> MPRYAMAID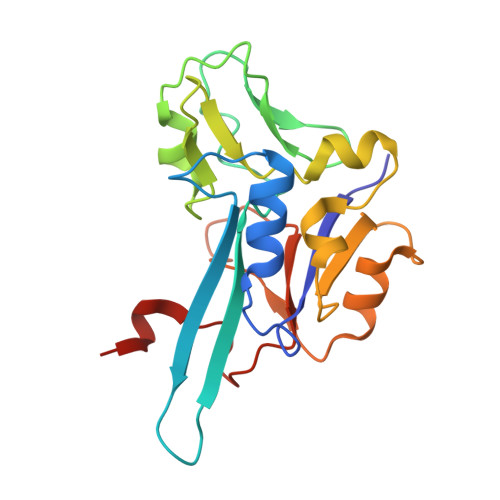LSLCVGCAACAVACKMENEVPPGVFNLWIREREVGEYPNLVVEFRPEQCLHCENPPCVPVCPTGASYQTKDGLVLVDPKKCIACGACIAACPYDARYLHPAGYVSKCTFCAHRLEKGKVPACVETCPTYCRTFGDLEDPESPVAKALKAAERVDVLRPEQGTRPKLFYLNAPSKKGLTRESEVHHG> MATHHTLWMGLALLGVLGDLQAAPEAQVSVQPNFQQDKFLGRWFSAGLASNSSWLREKKAALSMAKSV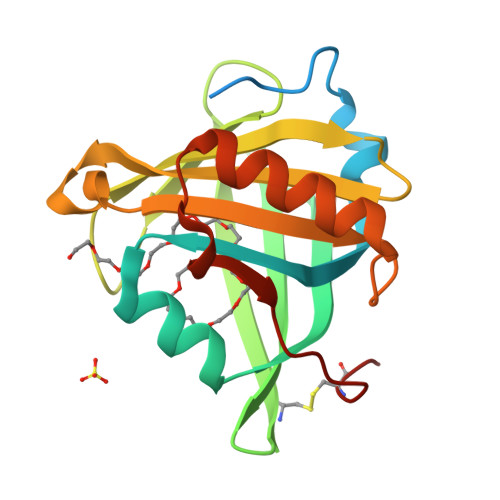VAPATDGGLNLTSTFLRKNQCETRTMLLQPAGSLGSYSYRSPHWGSTYSVSVVETDYDQYALLYSQGSKGPGEDFRMATLYSRTQTPRAELKEKFTAFCKAQGFTEDTIVFLPQTDKCMTEQ2-[(3-methoxybenzyl)amino]ethanesulfonic acid | C10 H15 N 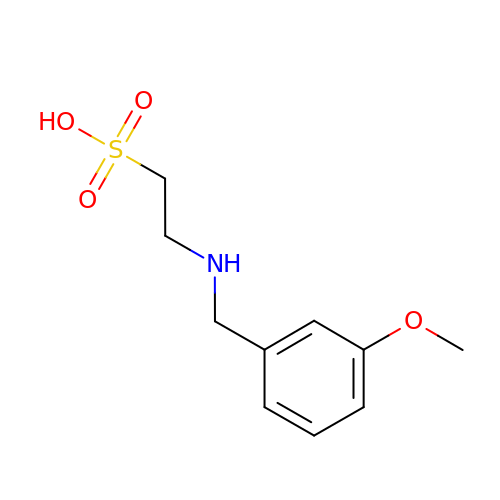O4 S | VKBJFTQAAOJIEB-UHFFFAOYSA-N> MLTRFRSAVLRGAVSITGARAASTAPVADHKGRVGHVSQVIGAVVDVHFADGVPPVLTALDVVDKLGRDEPLTLEIVQHLDAHTGRCIAMQTTDLLKLKAKVVSTGGNISVPVGRETLGRIFNVLGDAIDQRGPVGEKLRMPIHAVAPKLADQAAEDAVLTTGIKVIDLILPYCKGGKIGLFGGAGVGKTVIIMELINNVAKGHGGFSVFAGVGERTREGTDLYLEMMQSKVIDLKGESKCVLVYGQMNEPPGARARVAQSALTMAEYFRDVEGQDVLLFIDNIFRFTQANSEVSALLGRIPAAVGYQPTLAEDLGQLQERITSTTKGSITSVQAVYVPADDITDPAPATTFSHLDA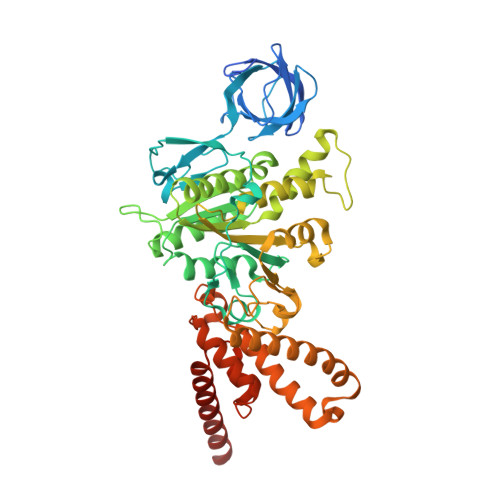TTVLDRAVAESGIYPAVNPLECASRIMDPDVISVDHYNVAQDVVQMLTKYRELQDIIAVLGIDELSEEDKLIVDRARKLVKFLSQPFQVAEVFTGMTGHYVQLDDTIDSFSGLLMGTYDQVPEMAFYMVGGINSVLEKAKKMAEEAAELEKMRRARVAQASS> MKG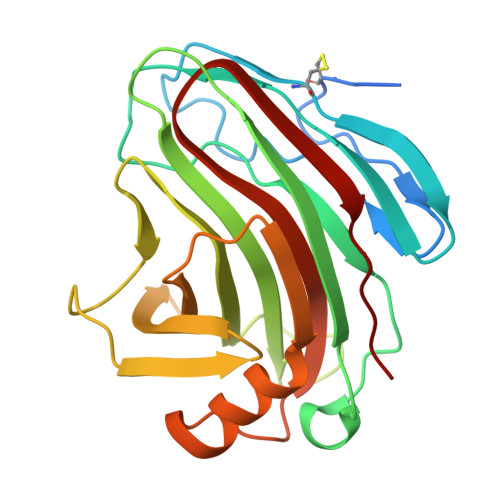FFAGVVAAATLAVASAGDYCGQWDWAKSTNYIVYNNLWNKNAAASGSQCTGVDKISGSTIAWHTSYTWTGGAATEVKSYSNAALVFSKKQIKNIKSIPTKMKYSYSHSSGTFVADVSYDLFTSSTASGSNEYEIMIWLAAYGGAGPISSTGKAIATVTIGSNSFKLYKGPNGSTTVFSFVATKTITNFSADLQKFLSYLTKNQGLPSSQYLITLEAGTEPFVGTNAKMTVSSFSAAVN>[8x]ARFEEQKLYIGGRYVEASSGATFETINPANGEVLAKVQRASREDVERAVQSAVEGQKVWAAMTAMQRSRILRRAVDILRERNDELAALETLDTGKPLAETRSVDIVTGADVLEYYAGLVPAIEGEQIPLRETSFVYTRREPLGVVAGIGAWNYPVQIALWKSAPALAAGNAMIFKPSEVTPLTALKLAEIYTEAGVPDGVFNVLTGSGREVGQWLTEHPLIEKISFTGGTSTGKKVMASASS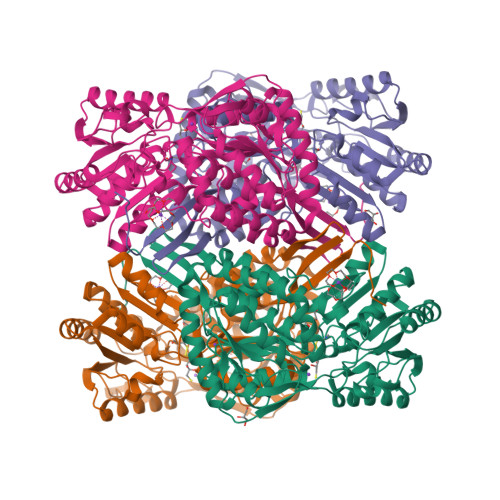SSLKEVTMELGGKSPLIIFPDADLDRAADIAVMANFFSSGQVCTNGTRVFIHRSQQARFEAKVLERVQRIRLGDPQDENTNFGPLVSFPHMESVLGYIESGKAQKARLLCGGERVTDGAFGKGAYVAPTVFTDCRDDMTIVREEIFGPVMSILVYDDEDEAIRRANDTEYGLAAGVVTQDLARAHRAIHRLEAGICWINTWGESPAEMPVGGYKQSGVGRENGLTTLAHYTRIKSVQVELGDYASVF2-azanyl-4-chloranyl-benzenecarbonitrile | C7 H5 Cl N2 | 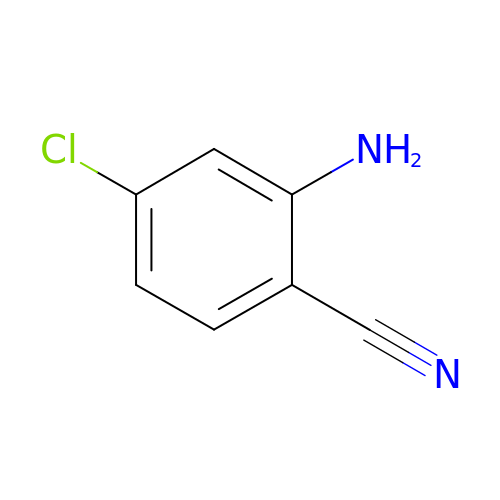UZHALXIAWJOLLR-UHFFFAOYSA-N> GSVKIGHYILGDTLGVGTFGKVKVGKHELTGHKVAVKILNRQKIRSLDVVGKIRREIQNLKLFRHPHIIKLYQVISTPSDIFMVMEYVSGGELFDYICK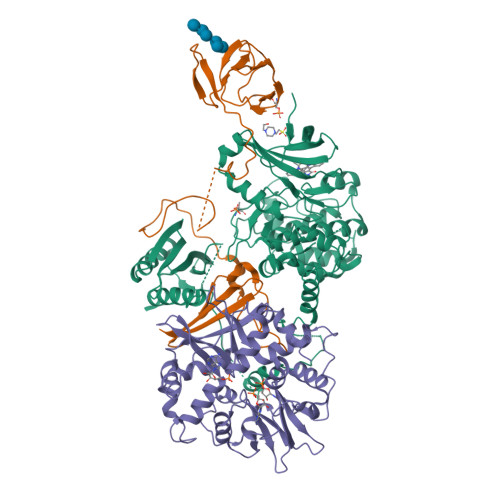NGRLDEKESRRLFQQILSGVDYCHRHMVVHRDLKPENVLLDAHMNAKIADFGLSNMMSDGEFLRTSCGSPNYAAPEVISGRLYAGPEVDIWSSGVILYALLCGTLPFDDDHVPTLFKKICDGIFYTPQYLNPSVISLLKHMLQVDPMKRASIKDIREHEWFKQDLPKYLFPEDPSYSSTMIDDEALKEVCEKFECSEEEVLSCLYNRNHQDPLAVAYHLIIDNRRIMNEAKDFYLATSPPDSFLDDHHLTRPHPERVPFLVAETPRARHTLDELNPQKSKHQGVRKAKWHLGIRSQSRPNDIMAEVCRAIKQLDYEWKVVNPYYLRVRRKNPVTSTYSKMSLQLYQVDSRTYLLDFRSIDDGITAAASGTATPQRSGSVSNYRSCQRSDSDAEAQGKSSEVSLTSSVTSLDSSPVDLTPRPGSHTIEFFEMCANLIKILAQ;> ARPTVIRWSEGGKEVFISGSFNNWSTKIPLIKSHNDFVAILDLPEGEHQYKFFVDGQWVHDPSEPVVTSQLGTINNLIHVKKSDFEVFDALKLDSMESSETSCRDLSSSPPGPYGQEMYAFRSEERFKSPPILPPHLLQVILNKDTNISCDPALLPEPNHVMLNHLYALSIKDSVMVLSATHRYKKKYVTTLLYKPI;> SNNSVYTSFMKSHRCYDLIPTSSKLVVFDTSLQVKKAFFALVTNGVRAAPLWDSKKQSFVGMLTITDFINILHRYYKSALVQIYELEEHKIETWREVYLQDSFKPLVCISPNASLFDAVSSLIRNKIHRLPVIDPESGNTLYILTHKRILKFLKLFITEFPKPEFMSKSLEELQIGTYANIAMVRTTTPVYVALGIFVQHRVSALPVVDEKGRVVDIYSKFDVINLAAEKTYNNLDVSVTKALQHRSHYFEGVLKCYLHETLETIINRLVEAEVHRLVVVDENDVVKGIVSLSDILQALVLTGG> ASVGGSLTGVGSIVTCLDSGRPGSIPCSKKWVLTLAVENGATAASSSVSATQAVYGSSSANATVRSADNPNTVYAFKYQVHITLTKSRIRLDYPLYYQSDFNNKPYEIVYKYNQKGPLNWLDNQCVATWGSSDPTCGYAYNPSWSTKPADRILYSQGFCCDCNAGDLLGLSPNRIRGGLDCSLLNFDNPTESAHCLRFDSLWYSAFQIGEPDVNFVILVNVTKCPLANSTIKSISGLVGNQDQAIQNCSTEIISLSPSSPIGYASNGKISAQAIGDFAPWEGTPSYSEKLFFVPSVCTDTSEAWCVDRISYIPTEINRWMLIDNDLVTITGDTCDKIGVSYSAFTNEGQRCERPTQSCLHDQLQDYYDSDLALEQTGKVGSYFVQFFGDFDVSGLTPRNPLLRFFTNRTQATEVVLQFAAEELFYTIYLAPARFLRHLSKINPFTSQSKGGLIDLWIVSEGTGQNAAQFTVSASCEPNVEPIQAQIVTLAPGQLVSISLPIIETKATGGAGVCNCTLRNALGQVLDVLVLEFNASSVHHHHHHHH

The protein HAP2/GCS1 (here called HAP2) is a gamete fusogen that is found in a wide range of eukaryotes including protists, algae, plants, insects, and hemichordates, and may be the “Eve” that enabled sex to evolve in early eukaryotes. Remarkably, HAP2 is structurally related to fusogens present in the membrane of enveloped viruses that allow them to fuse with and infect host cells. Although their sequences are highly divergent, HAP2 and viral class II fusogens have a common overall fold and domain arrangement. Here, we study the gamete fusogen HAP2 from Cyanidioschyzon merolae (Cyani), an extremophile red algae that grows at acidic pH at 45 °C. HAP2 has a trimeric postfusion structure with similarity to viral class II fusion proteins, but its prefusion structure has been elusive.

The Cyani HAP2 ectodomain (aa 28–564) was expressed in Drosophila S2 cells. A crystal structure of Cyani HAP2 to 2.3 Å resolution was solved by molecular replacement with the Chlamy postfusion HAP2 structure, and was refined to Rwork and Rfree values of 22.3 and 26.2%, respectively. Cyani HAP2 crystallizes as a monomer and has a rod-like shape with D3 in line with D2 and D1. It is much more extended than Chlamy HAP2, in which D3 folds back over D2 and D1 in the trimeric, postfusion state. Multi-angle light scattering (MALS) showed that Cyani HAP2 was monomeric in solution. PISA assembly analysis of the Cyani HAP2 crystal structure showed that no significant interactions with other monomers were present in the crystal lattice and thus that Cyani HAP2 was monomeric at high concentrations in crystals as well as in solution. The fusion loops of Cyani HAP2 locate to the membrane distal end of D2. Surprisingly, a β-sheet with three β-strands is present in D1 that is absent in the postfusion state of HAP2; we therefore term it the interim β-sheet. Although the interim β-sheet locates to the boundary of D1 with D3, it shares two backbone hydrogen bonds and an extensive hydrophobic interface with other residues in D1 and is therefore part of D1. Switching of the J0 β-strand from the interim β-sheet to the D1 β-sandwich in the postfusion state dictates a large change in orientation and position of D3 of HAP2, as the J0 β-strand leads directly into D3.>GQDMVSPPPPIADEPLTVNTGIYLIECYSLDDKAETFKVNAFLSLSWKDRRLAFDPVRSGVRVKTYEPEAIWIPEIRFVNVENARDADVVDISVSPDGTVQYLERFSARVLSPLDFRRFPFDSQTLHIYLIVRSVDTRNIVLAVDLEKVGKNDDVFLTGWDIESFTAVVKPANFALEDRLESKLDYQLRISRQYFSYIPNIILPMLFILFISWTAFWSTSYEANVTLVVSTLIAHIAFNILVETNLPKTPYMTYTGAIIFMIYLFYFVAVIEVTV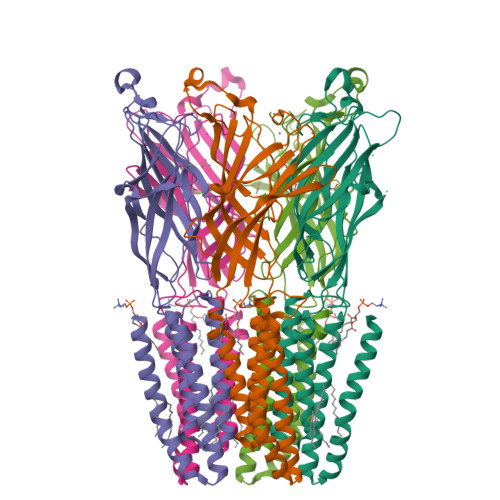QHYLKVESQPARAASITRASRIAFPVVFLLANIILAFLFFGF[5x]>[2x]NLLRRSGKRRRSESGSDSFSGSGGDSSASPQFLSGSVLSPPPGLGRCLKAAAAGECKPTVPDYERDKLLLANWGLPKAVLEKYHSFGVKKMFEWQAECLLLGQVLEGKNLVYSAPTSAGKTLVAELLILKRVLEMRKKALFILPFVSVAKEKKYYLQSLFQEVGIKVDGYMGSTSPSRHFSSLDIAVCTIERANGLINRLIEENKMDLLGMVVVDELHMLGDSHRGYLLELLLTKICYITRKSASCQADLASSLSNAVQIVGMSATLPNLELVASWLNAELYHTDFRPVPLLESVKVGNSIYDSSMKLVREFE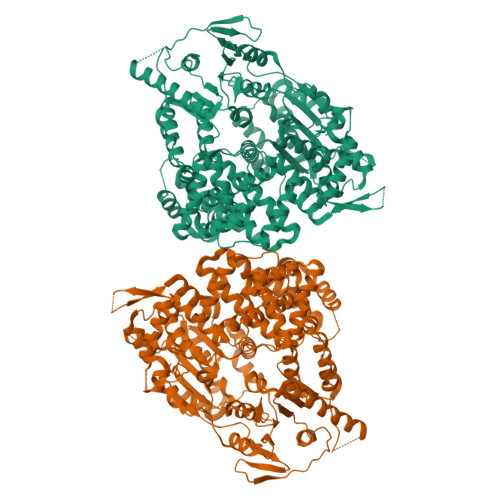PMLQVKGDEDHVVSLCYETICDNHSVLLFCPSKKWCEKLADIIAREFYNLHHQAEGLVKPSECPPVILEQKELLEVMDQLRRLPSGLDSVLQKTVPWGVAFHHAGLTFEERDIIEGAFRQGLIRVLAATSTLSSGVNLPARRVIIRTPIFGGRPLDILTYKQMVGRAGRKGVDTVGESILICKNSEKSKGIALLQGSLKPVRSCLQRREGEEVTGSMIRAILEIIVGGVASTSQDMHTYAACTFLAASMKEGKQGIQRNQESVQLGAIEACVMWLLENEFIQSTEASDGTEGKVYHPTHLGSATLSSSLSPADTLDIFADLQRAMKGFVLENDLHILYLVTPMFEDWTTIDWYRFFCLWEKLPTSMKRVAELVGVEEGFLARCVKGKVVARTERQHRQMAIHKRFFTSLVLLDLISEVPLREINQKYGCNRGQIQSLQQSAAVYAGMITVFSNRLGWHNMELLLSQFQKRLTFGIQRELCDLVRVSLLNAQRARVLYASGFHTVADLARANIVEVEVILKNAVPFKSARKAVDEEEEAVEERRNMRTIWVTGRKGLTEREAAALIVEEARMILQQDLVEM> MQYDDDWQYEDCKLARGGPPATIVAIDEESRNGTILVDNMLIKGTAGGPDPTIELSLKDNVDYWVLLDPVKQMLFLNSTGRVLDRDPPMNIHSIVVQVQCVNKKVGTVIYHEVRIVVRDRNDNSPTFKHESYYATVNELTPVGTTIFTGFSGDNGATDIDDGPNGQIEYVIQYNPEDPTSNDTFEIPLMLTGNVVLRKRLNYEDKTRYYVIIQANDRAQNLNERRTTTTTLTVDLE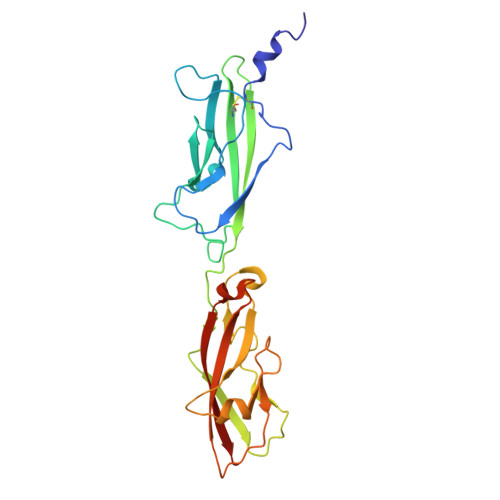HHHHHH>MNLTIPFAKGHATENDFIIIPDEDARLDLTPEMVVTLCDRRAGIGADGILRVVKAADVEGSTVDPSLWFMDYRNADGSLAEMCGNGVRLFAHWLYSRGLVDNTSFDIGTRAGVRHVDILQADQHSAQVRVDMGIPDVTGLSTCDINGQVFAGLGVDMGNPHLACVVPGLSASALADMELRAPTFDQEFFPHGVNVEIVTELEDDAVSMRVWERGVGETRSCGTGTVAAACAALADAGLGEG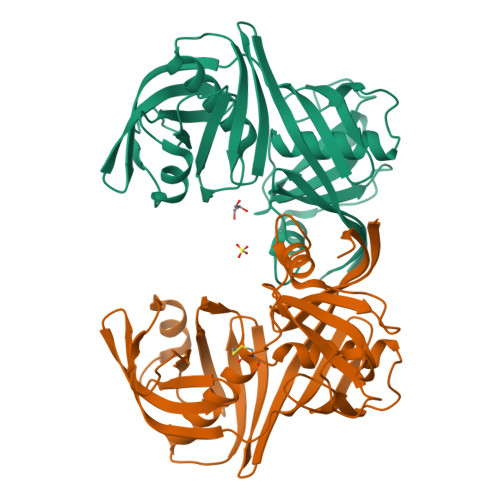TVKVCVPGGEVEVQIFDDGSTLTGPSAIIALGEVQIHHHHHH[2x]> MPVDFTGYWKMLVNENFEEYLRALDVNVALRKIANLLKPDKEIVQDGDHMIIRTLSTFRNYIMDFQVGKEFEEDLTGIDDRKCMTTVSWDGDKLQCVQKGEKEGRGWTQWIEGDELHLEMRVEGVVC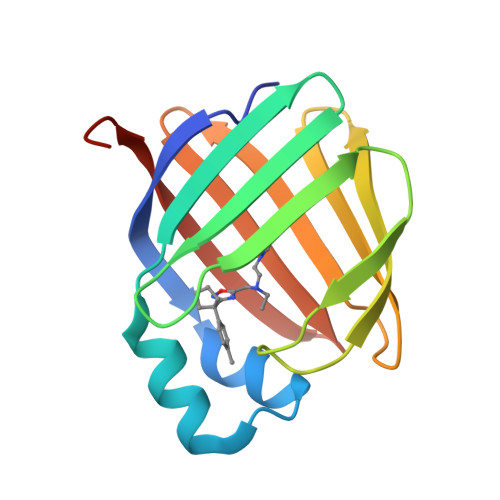KQVFKKVQHHHHHH>[4x]ASSQLIPNISPDSFTVAASTGMLSGKSHEMLYDAETGRKISQLDWKIKNVAILKGDISWDPYSFLTLNARGWTSLASGSGNMDDYAWMNENQSEWTDHSSHPATNVNHANEYDLNVKGWLLQDENYKAGITAGYQETRFSWTATGGSYS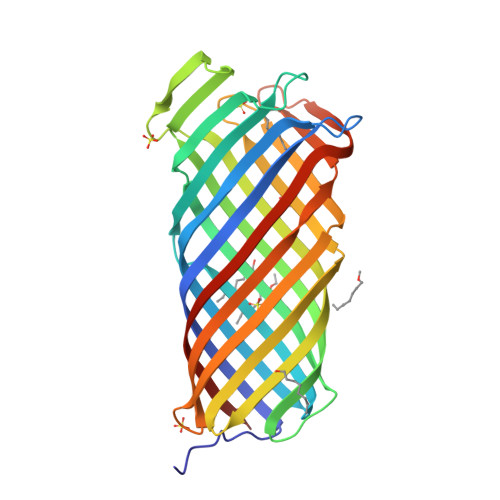YNNGAYTGNFPKGVRVIGYNQRFSMPYIGLAGQYRINDFELNALFKFSDWVRAHDNDEHYMRDLTFREKTSGSRYYGTVINAGYYVTPNAKVFAEFTYSKYDEGKGGTQTIDKNSGDSVSIGGDAAGISNKNYTVTAGLQYRFGGGGGG5,7-dihydroxy-2-(3-hydroxy-4-methoxyphenyl)-4H-1-benzopyran-4-one 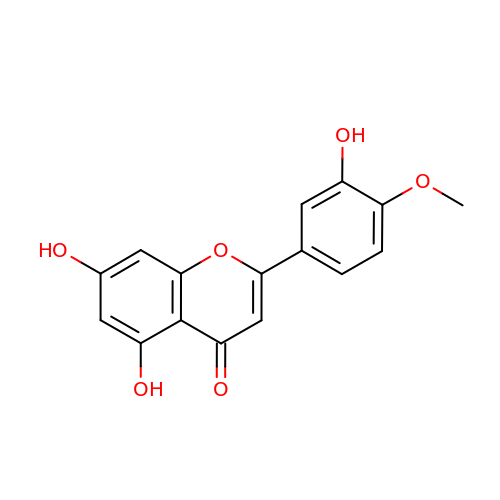| C16 H12 O6 | MBNGWHIJMBWFHU-UHFFFAOYSA-N> HPETLVKVKDAEDQLGARVGYIELDLNSGKILESFRPEERFPMMSTFKVLLCGAVLSRVDAGQEQLGRRIHYSQNDLVEYSPVTEKHLTDGMTVRELCSAAITMSDNTAANLLLTTIGGPKELTAFLHNMGDHVTRLDRWEPELNEAIPNDERDTTMPAAMATTLRKLLTGELLTLASRQQLIDWMEADKVAGPLLRSALPAGWFIADKSGAAERGSRGIIAALGPDGKPSRIVVI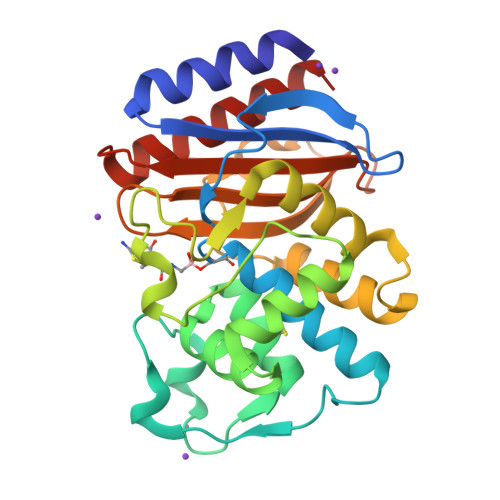YTTGSQATMDERNRQIAEIGASLIKHW>[2x]MPKLISSLFRNFTFKQYSLVCAMLFLGLQPVLGQFTIPEVPKEQTSVYDYAELLSAAEKASLENKLIKYSDTTSTQIVVVIIPS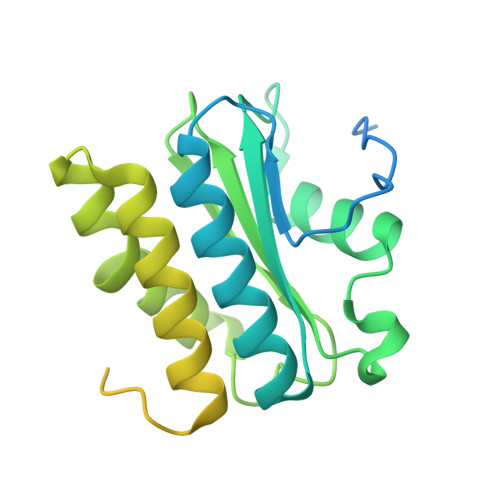TNGENINYLGAQWGEKWGIGQAKEDNGVLIILALNDKRIAINTGYGVEHLLTDAMSKRIIELDITPFFKRKDYPGGLDRGADAIFEVLTGEYQGSRQDNSEEGFPLGSLFFLVIIFIFILISTTKKGRGGDGGSGNKSGGFSFLDAIILSSMGRGNSSGGFGGSSGGGFGGGGGFGGGFGGGGFGGGGASGGW(1R,3S,4R)-3-[({3-hydroxy-2-methyl-5-[(phosphonooxy)methyl]pyridin-4-yl}methyl)amino]-4-methylcyclohexane-1-carboxylic acid | C16 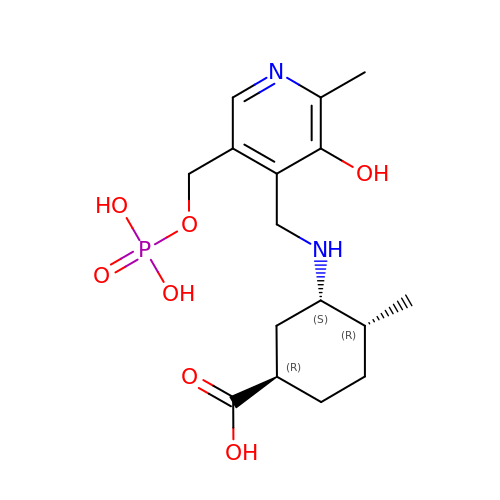H25 N2 O7 P | VMGXIUNFRDERKW-UDZFHETQSA-N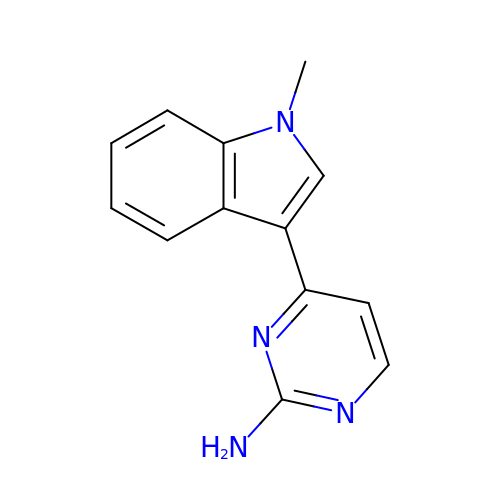4-(1-methylindol-3-yl)pyrimidin-2-amine | C13 H12 N4 | IEYXYKBZJHPKGV-UHFFFAOYSA-N2-{(1S)-1-[(6-chloro-3,3-dimethyl-3,4-dihydroisoquinolin-1-yl)amino]-2-phenylethyl}pyrido[4,3-d]pyrimidin-4(1H)-one | C26 H24 Cl N5 O | 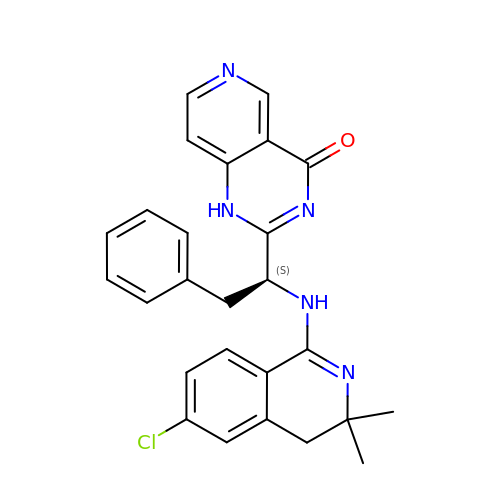DQYKHJYAOKSEPD-QFIPXVFZSA-N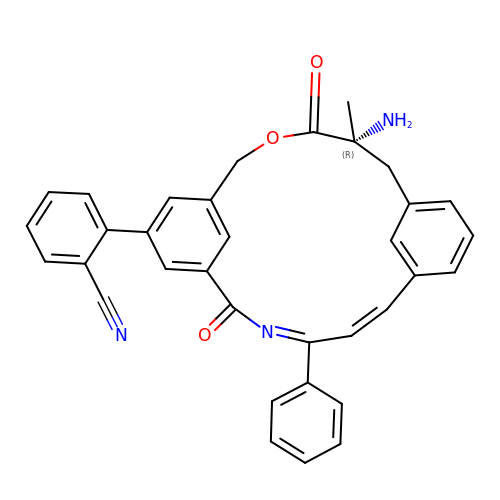2-[(5R)-5-amino-5-methyl-4,16-dioxo-14-phenyl-3-oxa-15-azatricyclo[15.3.1.1~7,11~]docosa-1(21),7(22),8,10,12,14,17,19-octaen-19-yl]benzonitrile | C34 H27 N3 O3 | GWSQLGYWQZHSHS-UUWRZZSWSA-N3-methyl-5-(2-phenylmethoxyphenyl)-4~{H}-1,2,4-triazole 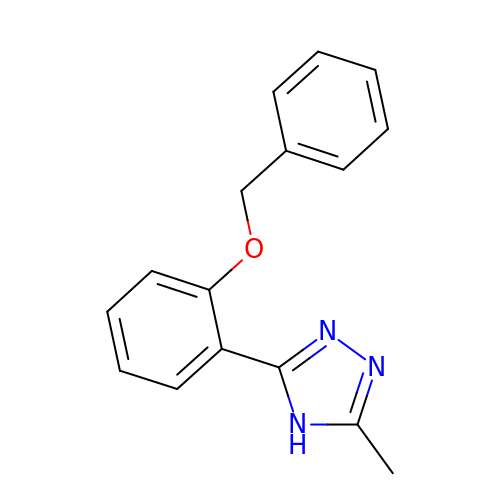| C16 H15 N3 O | NPTNHLPXAAOUPO-UHFFFAOYSA-N> SKSSQYRKMKTEWKSNVYLARSRIQGLGLYAARDIEKHTMVIEYIGTIIRNEVANRKEKLYESQNRGVYMFRMDNDHVIDATLTGGPARYINHSCAPNCV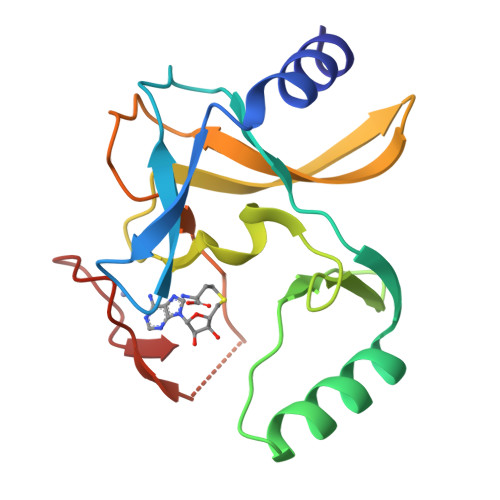AEVVTFERGHKIIISSSRRIQKGEELCYDYKFDFEDDQHKIPCHCGAVNCRKWM> SHMNAPAERAELTVPEMRQWLRNWVGKAVGK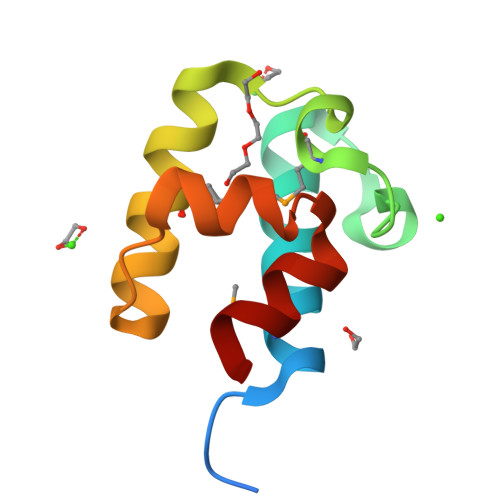APDSIDESVPMVELGLSSRDAVAMAADIEDLTGVTLSVAVAFAHPTIESLATRIIE>MNNMNVIIADDHPIVLFGIRKSLEQIEWVNVVGEFEDSTALINNLPKLDAHVLITDLSMPGDKYGDGITLIKYIKRHFPSLSIIVLTMNNNPAILSAVLDLDIEGIVLKQGAPTDLPKALAALQKGKKFTPESVSRLLEKISAGGYGDKRLSPKES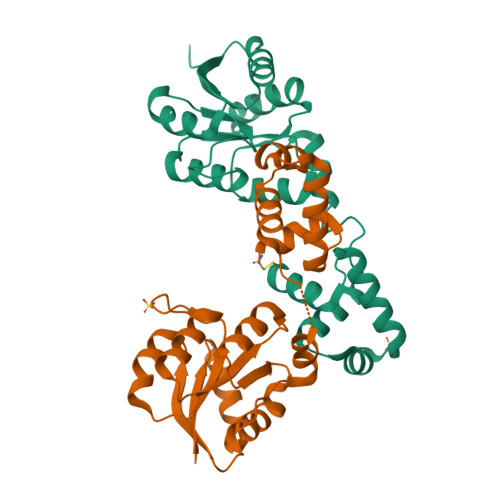EVLRLFAEGFLVTEIAKKLNRSIKTISSQKKSAMMKLGVENDIALLNYLSCVTL[2x]One peptidoglycan (PG) hydrolase, AtlA, has a predominant role in E. faecalis septum cleavage. atlA mutants are viable but form extremely long chains and are greatly attenuated in the zebrafish virulence model of infection. AtlA is a multimodular N-acetylglucosaminidase belonging to the glycoside hydrolase GH73 family in the CAZy (Carbohydrate-Active enZYmes Database). The enzyme undergoes post-translational modifications (glycosylation and proteolytic cleavage) and preferentially binds to denuded glycan chains (preferentially found at the midcell) via the C-terminal LysM domain.

The structure of the catalytic domain of AtlA (AtlAc) (161 residues) was solved at a resolution of 1.45 Å. It adopts a lysozyme α/β fold with an α-lobe containing five α-helices (α1: 180–197, α2: 202–213; α3: 265–278, α4: 299–306, and α5: 315–327), five helices 310, a small β-hairpin, and a major β-lobe covering the binding site, made of two antiparallel β-strands (β1: 239–248, β2: 251–260) connecting α2 and α3. The structure also contains five glycerol molecules coming from the cryogenic buffer. Only one polypeptide of AtlAc is found in the asymmetric unit, suggesting that the protein is monomeric in solution. The AtlAc active site shows two highly conserved glutamate residues: E212 is equivalent to L. monocytogenes Auto E122 and FlgJSt E184 catalytic residues and is located at a similar position, at the end of helix α1. The second predicted catalytic glutamate, E246, stands on β2 and is equivalent to E156 in L. monocytogenes Auto and E223 in FlgJSt. Unlike Auto and FlgJSt, which show an open groove for the active site, the AtlAc active site shapes into a tunnel. The β-hairpin closing on the α-lobe by forming several hydrogen bonds: E246 OE2 on strand β1 with K232 NZ on a loop between α2 and β1, E246 with T312 OG1 and the water molecule 12 (Wat12), and T312 OG1 with Y247 main chain N. The crystal structure of AtlAc revealed a partial occlusion of the catalytic tunnel by the K232 residue. In AtlAc, the β-hairpin shows a “closed” conformation and the distance between E212 and E246 is 9 Å, which is the distance required for a classic type 2 nucleophile substitution with an inverting mechanism.

> MGSALSPTQSPSEFIAELARCAQPIAQANDLYASVMMAQAIVESGWGASTLSKAPNYNLFGIKGSYNGQSVYMDTWEYLNGKWLVKKEPFRKYPSYMESFQDNAHVLKTTSFQAGVYYYAGAWKSNTSSYRDATAWLTGRYATDPSYNAKLNNVITAYNLTQYDTPSSGSHHHHHH Sirtuins are NAD+-dependent protein lysine deacylases that sense the cellular nutrient status, regulate energy metabolism and stress responses, and have been implicated in aging processes and aging-related diseases. Sirtuins feature differing substrate acyl selectivities. Here, we analyse modulation of Sirt6 and other isoforms by quercetin and its derivatives in activity and binding assays and through crystal structure analyses of modulator complexes of Sirt6 and Sirt2. Our results hence reveal sites and mechanisms for Sirtuin modulation by quercetin derivatives and provide helpful insights for Sirt6 modulator development.

Quercetin caused a concentration-dependent inhibition of all Sirtuin isoforms except for Sirt6, which was instead activated. Due to the lack of a Sirt6-like binding site in the other isoforms, quercetin has to exploit an alternative binding site to cause this opposite, inhibitory effect. To identify the alternative quercetin binding site and modulation mechanism, we determined a crystal structure of a Sirt2/quercetin complex at 2.2 Å resolution. Well-defined electron density revealed that quercetin binds at the Sirt2 active site entrance, through π-π stacking with Tyr-114 and Phe-235 and anion–π interactions with Glu-116 and Glu-120. Interestingly, quercetin is located between two symmetry-related Sirt2 monomers and interacts with the same surface region of the second monomer, albeit with rotated orientation and through fewer contacts, suggesting the interaction with the first monomer to be the one relevant in solution. An overlay with a Sirt2/substrate peptide complex reveals that quercetin partly occupies the pocket accommodating substrate moieties C-terminal from the acetyl-Lys and thus sterically prevents substrate binding. Such a peptide competitive mechanism is supported by Sirt2 inhibition tests that show that increasing substrate concentrations lead to weaker inhibitory effects of a fixed inhibitor concentration. Comparing the Sirt2/quercetin complex to other Sirtuin isoforms reveals that its binding site is also accessible in Sirt1, 3, and 5, whereas it is occupied in Sirt6 by the N-terminus. Since the quercetin binding site of Sirt6 is blocked in these other isoforms, our structures define two mutually exclusive modulator binding sites for Sirt6 and for Sirt1,2,3,5, respectively.

>[2x]HMKERLLDELTLEGVARYMQSERCRRVICLVGAGISTSAGIPDFRSPSTGLYDNLEKYHLPYPEAIFEISYFKKHPEPFFALAKELYPGQFKPTICHYFMRLLKDKGLLLRCYTQNIDTLERIAGLEQEDLVEAHGTFYTSHCVSASCRHEYPLSWMKEKIFSEVTPKCEDCQSLVKPDIVFFGESLPARFFSCMQSDFLKVDLLLVMGTSLQVQPFASLISKAPLSTPRLLINKEKAGQSDPFLGMIMGLGGGMDFDSKKAYRDVAWLGECDQGCLALAELLGWKKELEDLVRREHASIDAQS(13-oxo-9(Z),11(E),15(Z)-octadecatrienoic acid) | 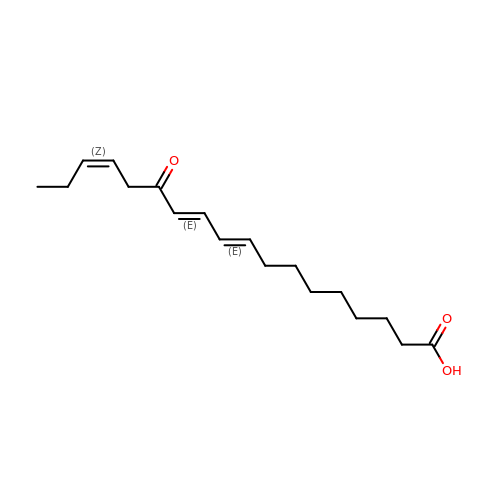C18 H28 O3 | BNMYUQILBYIYOG-GLVBUJDASA-N Gaucher disease (GD) is the most common lysosomal storage disorder which is caused by inherited deficiencies in β‐glucocerebrosidase (glucosylceramidase, GCase, GBA, EC 3.2.1.45). GBA is primarily responsible for catalyzing the degradation of GlcCer by hydrolytic cleavage of the β‐glucose moiety from the aglycone to yield free ceramide and glucose. This is achieved with retention of β‐anomeric stereochemistry of the released glucose unit through a Koshland double displacement mechanism using Glu340 as the catalytic nucleophile and Glu235 as the catalytic acid‐base. Here, we report the design, synthesis, and structural analysis of a range of cyclophellitol epoxide and aziridine inactivators and activity‐based probes (ABPs) for human β‐glucocerebrosidase (GBA).

In addition to a previously reported structure of rhGBA in complex with the O6−Cy5 tagged cyclophellitol epoxide ABP 9, a serendipitous co‐complex of O6−BODIPY tagged ABP 5 and N‐acyl aziridine 3 was obtained in this study by accidental soaking of rhGBA crystals in complex N‐acyl aziridine 3 with additional ABP 5. In the resulting co‐complex, clear electron density was observed for 3 bound covalently to Glu340, with its ring‐opened N‐acyl chain bound in the narrow active site cavity flanked by Gln283 and Tyr313. Additionally, unambiguous electron density for an intact molecule of ABP 5 was observed, allowing the full ABP to be modelled at the surface of molecule A of the crystallographic dimer. Specifically, the BODIPY tag binds at the dimer interface in a hydrophobic cavity formed by Leu241, Tyr244, Pro245, Phe246 and Tyr313, which we reported previously to accommodate the Cy5 tag of ABP 9. The unreacted cyclophellitol of 5 sits exposed at the surface of the protein, making no hydrogen bonding interactions with the enzyme; however, the hydrophobic face of the cyclophellitol unit lies above the exposed side chain of Leu241. Whilst the binding of ABP 5 could be considered artefactual, it is notable that very simple torsional rotation of the linker allows the linker and cyclophellitol unit to be placed in the active site, putting the epoxide warhead in perfect super‐position with the trapped aziridine without any movement of the BODIPY group itself. In combination with the previously reported structure of rhGBA in complex with a Cy5 tagged ABP 9, this ABP 5 co‐complex provides further evidence for a unique binding mode of this hydrophobic cavity, which has recently been exploited for the binding of a novel class of pyrrozopyrazine activators with chaperoning potential. Considering these preferences and the structural information provided by the co‐complex of 3 and 5, we suggested that binding of the O6‐substituent and aziridine N‐functionalization are structurally exclusive and may reflect the enzymes specificity for a lipid substrate with two acyl tails.

>[2x]ARPCIPKSFGYSSVVCVCNATYCDSFDPPTFPALGTFSRYESTRSGRRMELSMGPIQANHTGTGLLLTLQPEQKFQKVKGFGGAMTDAAALNILALSPPAQNLLLKSYFSEEGIGYNIIRVPMASCDFSIRTYTYADTPDDFQLHNFSLPEEDTKLKIPLIHRALQLAQRPVSLLASPWTSPTWLKTNGAVNGKGSLKGQPGDIYHQTWARYFVKFLDAYAEHKLQFWAVTAENEPSAGLLSGYPFQCLGFTPEHQRDFIARDLGPTLANSTHHNVRLLMLDDQRLLLPHWAKVVLTDPEAAKYVHGIAVHWYLDFLAPAKATLGETHRLFPNTMLFASEACVGSKFWEQSVRLGSWDRGMQYSHSIITNLLYHVVGWTDWNLALNPEGGPNWVRNFVDSPIIVDITKDTFYKQPMFYHLGHFSKFIPEGSQRVGLVASQKNDLDAVALMHPDGSAVVVVLNRSSKDVPLTIKDPAVGFLETISPGYSIHTYLWHRQ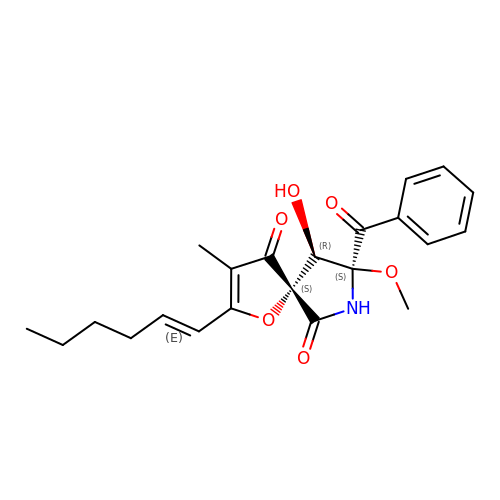(5~{S},8~{S},9~{R})-2-[(~{E})-hex-1-enyl]-8-methoxy-3-methyl-9-oxidanyl-8-(phenylcarbonyl)-1-oxa-7-azaspiro[4.4]non-2-ene-4,6-dione | C22 H25 N O6 | WDHGEYIVJHPIOB-HVQJOPHCSA-N> MNHKVHHHHHHIEGRHMPHILTIKHKRGKPGAVYYPLQLKAVPKPGPPGPGEVLIRMAAAALNHRDHFIRQHLYPNISFESPLFSDACGTVVEVGPGCK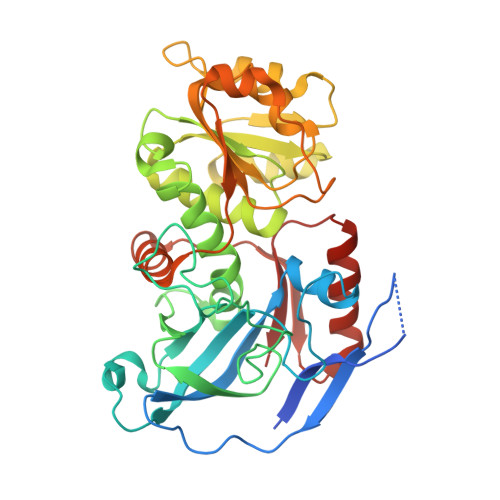RSDELLNKLVVLVPYRGWDGDSPDGPEDWSAFATVGGTEPYRTLGGGQTWMVAAEDQVEVCPPHLSAVEGAALPSCGVTAWRALVTKCGRANVGPGRNILITGIGGGVALQALQMALALGANVYVTSGSEAKLARARQLGAKGGALYTEQDWPKIIAGLLPLAHPLLDAIVDGAGGDIVIRAVPILKPGGVIAIYGMTTAPVLDWPMQAVLKNIELRGTTLGSRAEFRDMVAFVAEHKLRPVISRTVKGLDCVDAIDGLFEDLKGGKQFGKLVIEI>MSNEIPKPVAPAPDILRCAYAELVVTDLAKSRNFYVDVLGLHVSYEDENQIYLRSFEEFIHHNLVLTKGPVAALKAMAFRVRTPEDVDKAEAYYQELGCRTERRKDGFVKGIGDALRVEDPLGFPYEFFFETTHVERLHMRYDLYSAGELVRLDHFNQVTPDVPRGRKYLEDLGFRVTEDIQDDEGTTYAAWMHRKGTVHDTALTGGNGPRLHHVAFSTHEKHNIIQICDKMGALRISDRIERGPGRHGVSNAFYLYILDPDNHRIEIYTQDYYTGDPDNPTITWNVHDNQRRDWWGNPVVPSWYTEASKVLDLDGNVQEIIERTDDSELEVTIGADGFSFTRAGDEDGSYHGQ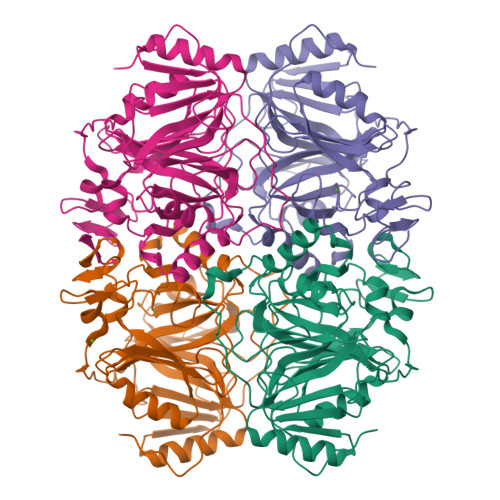ASKGFKLGNQL[4x]> DA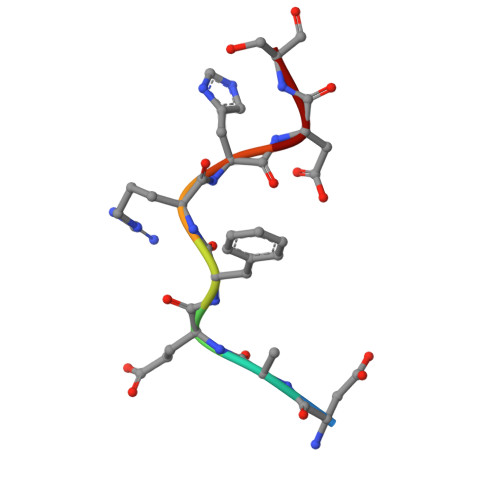EFRHDS>[4x]LPRETDEEPEEPGKKGSFVEMVDNLRGKSGQGYYVEMTVGSPPQTLNILVDTGSSNFAVGAAPHPFLHRYYQRQLSSTYRDLRKGVYVPYTQGKWEGELGTDLVSIPHGPNVTVRANIAAITESDKFFINGSNWEGILGLAYAEIARPDDSLEPFFDSLVKQTHVPNLFSLQLCGAGFPLNQSEVLASVGGSMIIGGIDHSLYTG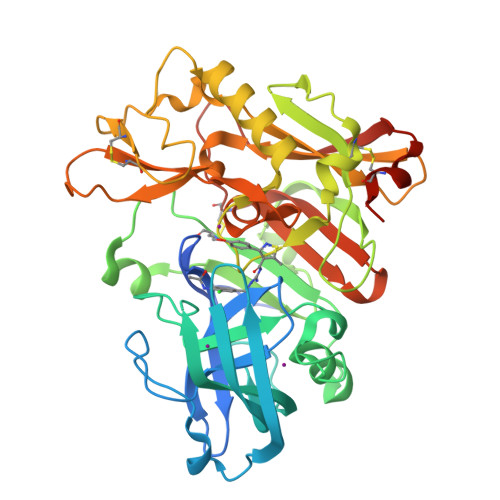SLWYTPIRREWYYEVIIVRVEINGQDLKMDCKEYNYDKSIVDSGTTNLRLPKKVFEAAVKSIKAASSTEKFPDGFWLGEQLVCWQAGTTPWNIFPVISLYLMGEVTNQSFRITILPQQYLRPVEDVATSQDDCYKFAISQSSTGTVMGAVIMEGFYVVFDRARKRIGFAVSACHVHDEFRTAAVEGPFVTLDMEDCGYNIPQTDEST3-(4-AMINO-2-METHYL-PYRIMIDIN-5-YLMETHYL)-5-(2-HYDROXY-ETHYL)-4-METHYL-THIAZOL-3-IUM 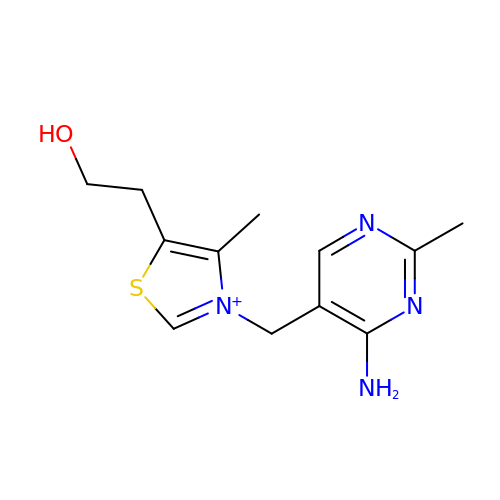| C12 H17 N4 O S | JZRWCGZRTZMZEH-UHFFFAOYSA-N> GRARKLCSLDNGDCDQFCHEEQNS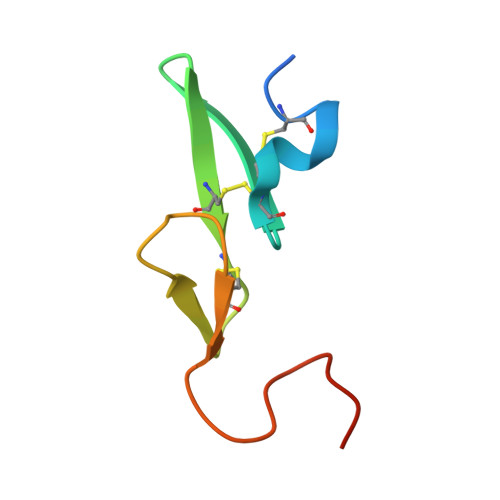VVCSCARGYTLADNGKACIPTGPYPCGKQTLER1-(4-(3-methylbenzyl)-3,4-dihydroquinoxalin-1(2H)-yl)ethanone | C18 H20 N2 O | 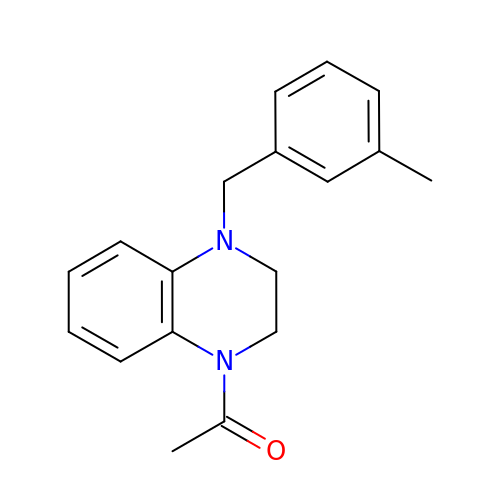GJDUNGUDLCUYKF-UHFFFAOYSA-N> GSHMSSLPVPYKLPVSLSVGSCVIIKGTPIHSFINDPQLQVDFYTDMDEDSDIAFHFRVHFGNHVVM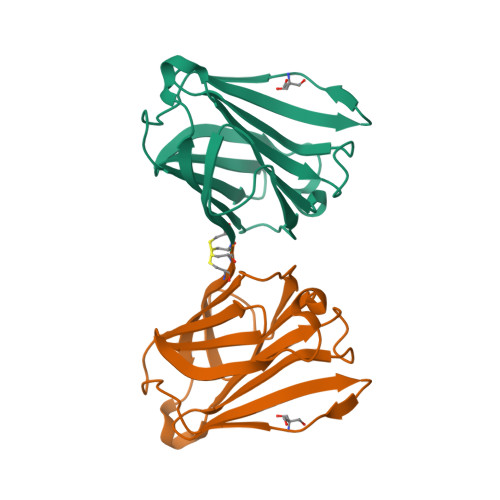NRREFGIWMLEETTDYVPFEDGKQFELCIYVHYNEYEIKVNGIRIYGFVHRIPPSFVKMVQVSRDISLTSVCVCN>MASAVAVPMDSTGPYRTVSHPENAPSGVDAGVGPSEWTHAYANPAHNAAFPVPDDAPEWIRNGVSWLFPEARAWPLANPPFGSKTYGAAEASVTQTQFYGNALGPSVVDGVVYAESDDMFAYAVNAKTGKLIWRASPVGNNLMGNPLVIGNTVYLSAGSVAFNFANVLRYAHNPSASARGLNVSFNGIYALNRSNGKLLWYFATPGETMATPAYDNNTLFIADGAGNAFGINATTGKQVWKTHVGGMDNMSSVTAYRHNIYFAMAIKPYLYCLNESNGHIVWKGTIPGASNTGIGDVSPAAADGVVVLDATTKPQANKKAMFSNVIRAFDAKTGAVLWTRNMGSGGKIPAFKGGVPMIHNNIVYVGNPVASTYQAYELKTGKLLWTWHVPTKVAAGAGRSAPTYYKGLLYITTGQYIFVVNPATGKELHQHHIGGQFGIESPVIVGGTVYLTNSWDWIM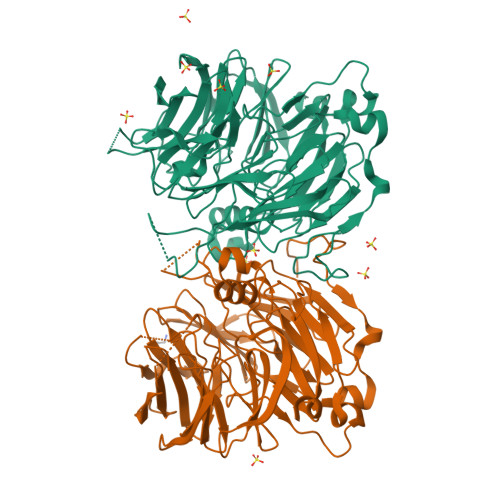AIPLKTISHGS[6x]> DPSRIPSALIGRPAPQTALPPLEGLQADNVQVPGLDPAAFKGKVSLVNVWASWCVPCHDEAPLLTELGKDKRFQLVGINYKDAADNARRFLGR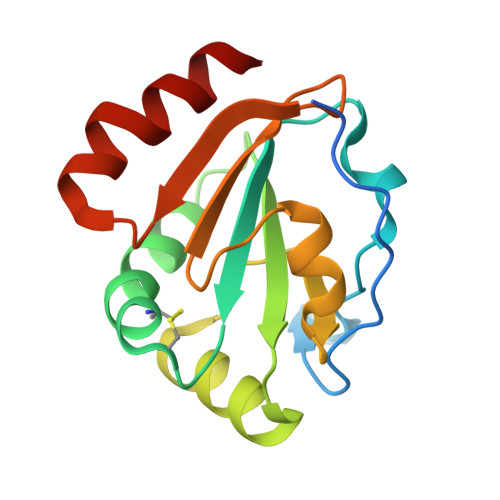YGNPFGRVGVDANGRASIEWGVYGVPETFVVGREGTIVYKLVGPITPDNLRSVLLPQMEKALK methyl hydrogen 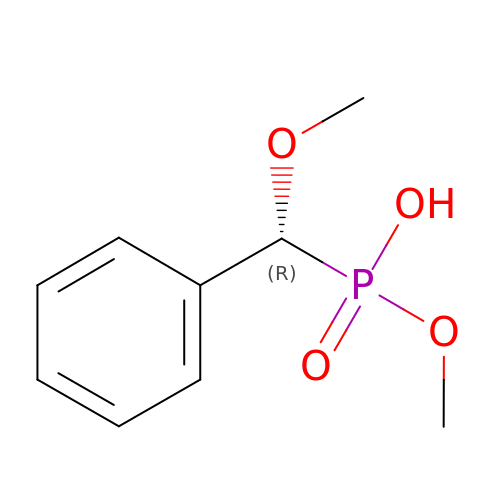(R)-[(R)-methoxy(phenyl)methyl]phosphonate | C9 H13 O4 P | YPAATCUNRIAADK-SECBINFHSA-N>[2x]MENTNLRTKTLRDGTTAEELFSQDGLSFNDFIILPGFIDFDSSKVNVSGQFTKNILLHLPLVSSPMDTVTESSMARAMALMGGIGVIHNNCTVEQQARMVRSVKLYRNGFIMKPKSVSPDVPVSTIRNIKSEKGISGILVTEGGKYDGKLLGIVCTKDIDFVKDASAPVSQYMTRRENMTVERYPIKLEEAM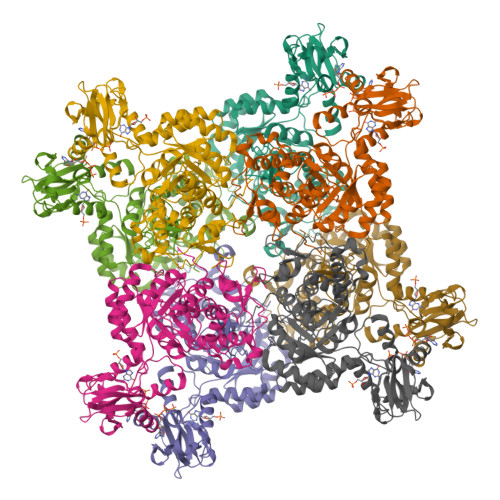DVLNRSRHGYLPVLNDKDEVVCLCSRRDAVRARDYPNSSLDRNGHLLCAAATSTREADKGRVAALSEAGIDVLVLDSSQGNTIYQVSFIRWVKKTYPHLEVVAGNVVTQDQAKNLIDAGADSLRIGMGSGSICITQEVLACGRPQATAIYKVARYAASRGVPCVADGGLRNVGDVCKALAVGANVAMLGSMIAGTSETPGEYFFKDGMRLKGYRGMGSIDAMLQGRESGKRYLSENETLQVAQGVAGAVLDKGSVLKLLAYIHKGLQQSAQDIGEVSFDAIREKVYEGQVLFNRRTLTAQSEGAVHSLHHYERKLFASKL Tandem pore domain (K2P) potassium channels modulate resting membrane potentials and shape cellular excitability. For the mechanosensitive subfamily of K2Ps (including the TREK1, TREK2, and TRAAK channels), diverse stimuli control channel activity, including lipids, pH, heat, membrane tension, post-translational modification, and an array of pharmacologically active agents including volatile anesthetics, antidepressants, and neuroprotective agents. Two key regions of the mechanosensitive K2P channel structure appear to control channel function, the conformationally flexible TM4 helix, and the selectivity filter. Overall, this cryo-EM structure exhibits K2P architectural features consistent with prior crystallographic studies: a dimeric channel assembly with each subunit composed of four transmembrane helices, a domain-swapped cap located above the selectivity filter, and an extended membrane facing TM2/TM3 loop within each subunit.

In the POPA structure, both TM4 are in the “up” conformation (d) and the membrane facing fenestration is closed (e). There are two POPA binding sites where the lipid density interacts directly with the core of the protein. At the upper site (d, e), the cryo-EM density for a lipid acyl tail can be seen inserting itself underneath TM4 to sit behind the selectivity filter pore helices. We find that the presence of a lipid tail in the upper binding site forces an inward reorientation of the W275 sidechain toward the core of the protein, moving it closer to the G137 residue. Our structures suggest that a lipid bound at this upper site may similarly “bypass” the influence of the TM4 helix position to directly modulate the TREK1 selectivity filter. The POPA density located at the lower binding site is positioned between the TM4 and TM1 helices, such that this binding site is only constituted when TM4 approaches TM1 in the “up” state and is broken in the TM4 “down” state. An array of basic residues from both TM4 and TM1 surround the negatively charged headgroup of the PA lipid, suggesting a clear electrostatic basis for the binding of PA and other anionic lipids at this site. The S300 residue, a protein kinase C phosphorylation target in the proximal C-terminus of TREK144, lies directly in the center of the lower POPA binding site, 4.8 Å away from the well-resolved POPA headgroup. In this location, phosphorylation of S300 would be predicted to create both electrostatic and steric clashes with the headgroup of a bound anionic lipid and would disfavor the anionic lipid bound TM4 “up” state.

>MAAPDLLDPKSATHNTKPRLSFSSKPIVYNSGDDCESITTVMKWKTVLAIFLLVVLYLIIGATVFKALEQPEEGLQKYRIIQEKIDFLSMHTCVQTSELEDLVKQVVLAIRAGVNPSGHPSQESSMWDLSSSFFFAGTVITTIGFGNVSPHTEGGRIFCIIYALLGIPLFGFLLAGVGDQLGTIFGKGIAKVEKMFVKWNVSQTKIRVTSTVLFILFGCLLFVALPALIFQHIEGWSALESIYFVVITLTTIGFGDFVAGGSEIEYLDYYKPIVWFWILVGLAYFAAVLSMIGDWLRVISKKTKEEVGEFRAHAAEWTANV[2x]The microscopic openings across the walls of many capillaries contain a protein mesh that is formed by the extracellular domain (ECD) of plasmalemma vesicle-associated protein (PLVAP). Current evidence suggests that a single transmembrane protein, plasmalemma vesicle-associated protein (PLVAP or PV1), constitutes the diaphragm’s sole structural protein. PLVAP is a type II transmembrane protein of ~60 kDa with an ~390-amino acid C-terminal extracellular domain (ECD), a single transmembrane domain, and a 26-amino acid N-terminal cytoplasmic domain. The three-dimensional structure of PLVAP CC1 presented here shows that it forms a parallel disulfide-bonded dimeric coiled coil.

PLVAP CC1 crystallized in the I212121 space group with unit-cell parameters 33.8 Å, 89.0 Å, and 180.9 Å, referred to hereafter as crystal form II. X-ray diffraction data were collected and processed to 1.95 Å. Because PLVAP CC1 contains only one methionine, we initially produced PLVAP CC1 with selenium-labeled methionine (SeMet) for multi- or single-wavelength anomalous diffraction (MAD or SAD). However, the resulting anomalous signals were too weak to be useful for structure determination. The PLVAP CC1 dimer model from crystal form I was used to determine the structure of PLVAP CC1 in crystal form II by MR. The electron density for residues 141 to 145 of crystal form II chain B was not visible. Structure-based analysis by the Socket2 algorithm for both crystal forms shows that most of the PLVAP CC1 dimer exhibits a classical coiled-coil configuration characterized by heptad repeats (abcdefg in Fig. 6A). Among PLVAP CC1 dimers, the average rmsds are 1.15 Å for crystal form I chain A + B vs. chain C + D, 0.89 Å for crystal form I chain A + B vs. crystal form II chain A + B, and 0.84 Å for crystal form I chain C + D vs. crystal form II chain A + B. Conformational differences are greatest at the N terminus.

>[2x]GPGTSRQCQEQLKEVNKTCEALLFKLGEKVKTLEMEVAKEKAVCSKDKESLLAGKRQTEEQLEACGKARERQQQEQQVTEENLRKVQSLCIPLDQ~{N}-(3-chloranyl-4-methoxy-phenyl)-7-(3,4-dimethylphenyl)pyrrolo[2,3-d]pyrimidin-4-amine 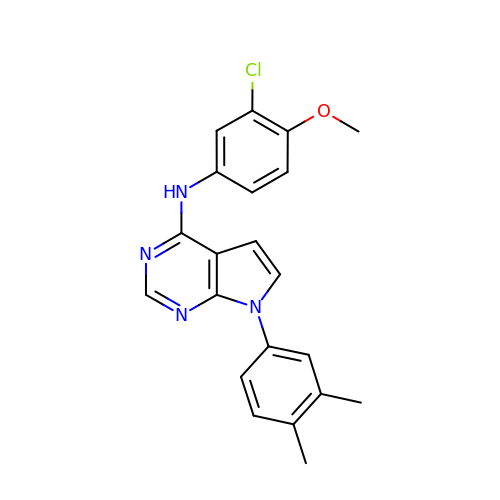| C21 H19 Cl N4 O | DZIHITUUUPJMOQ-UHFFFAOYSA-N>[8x]GKLEARAALNQALEMKRQGKREKAQKLFMHALKMDPDFVDALTEFGIFSEEDKDIIQADYLYTRALTISPYHEKALVNRDRTLPLVEEIDQRYFSIIDSKVKKVMSIPKGNSALRRVMEETYYHHIYHTVAIEGNTLTLSEIRHILETRYAVPGKSLEEQNEVIGMHAAMKYINTTLVSRIGSVTISDVLEIHRRVLGYVDPVEAGRFRTTQVLVGHHIPPHPQDVEKQMQEFVQWLNSEEAMNLHPVEFAALAHYKLVYIHPFIDGNGRTSRLLMNLILMQAGYPPITIRKEQRSDYYHVLEAANEGDVRPFIRFIAKCTETTLDTLLFATTEYSVALPEAQP

AMPylation (or adenylylation) is the transfer of AMP from ATP to a Tyr or Thr/Ser residue in target proteins. Interestingly, in eukaryotic genomes only one FIC-domain containing protein has been identified to date, HYPE or FICD, and it is strongly conserved from C. elegans to humans. Here we describe the first crystal structure of a eukaryotic HYPE encompassing the two TPR-motifs, an α-helical linker, and the FIC domain of the human protein. We demonstrate that HYPE forms stable dimers with structurally and functionally integrated FIC-domains and with TPR-motifs exposed for protein-protein interactions.

The structure of HYPE E234G with the nonhydrolysable ATP analog, APCPP, shows a different position of the α-phosphate that would be incompatible with catalysis, suggesting that APCPP is not a physiological ATP mimic in this case. However, the basal activity of the wild-type HYPE is probably lower when compared to the E234G variant. It has been previously documented that the proposed intramolecular inhibition in several FIC domains (Engel et al., 2012) can be reversed by replacing the critical inhibitory Glu residue by Gly, using autoAMPylation as a readout (Goepfert et al., 2013). A Mg2+ ion is visible in the E234G variant of HYPE; it bridges the α- and β-phosphates and is coordinated by the conserved Asp367 side chain.> GASIVSLLGIKVLNNPAKFTDPYEFEITFECLESLKHDLEWKLTYVGSSRSLDHDQELDSILVGPVPVGVN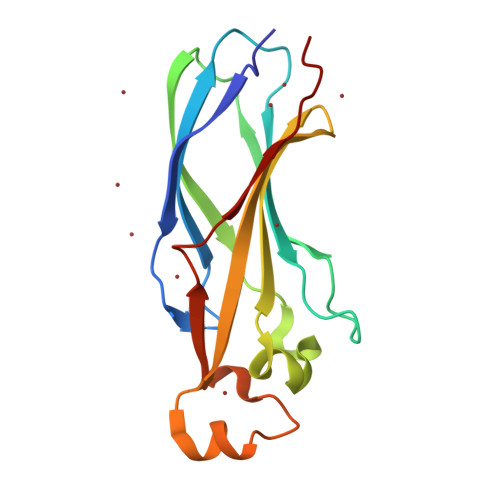KFVFSADPPSAELIPASELVSVTVILLSCSYDGREFVRVGYYVNNEYDEEELRENPPAKVQVDHIVRNILAEKPRVTRFNIVWD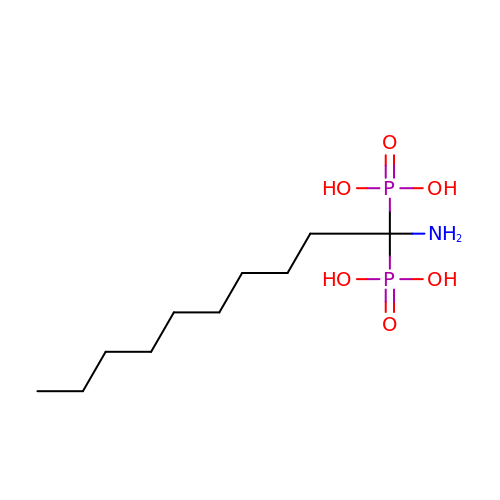(1-azanyl-1-phosphono-decyl)phosphonic acid | C10 H25 N O6 P2 | TWYYYYAFACTHMV-UHFFFAOYSA-N>GEIRPTIGQQMETGDQRFGDLVFRQLAPNVWQHTSYLDMPGFGAVASNGLIVRDGGRVLVVDTAWTDDQTAQILNWIKQEINLPVALAVVTHAHQDKMGGMDALHAAGIATYANALSNQLAPQEGMVAAQHSLTFAANGWVEPATAPNFGPLKVFYPGPGHTSDNITVGIDGTDIAFGGCLIKDSKAKSLGNLGDADTEHYAASARAFGAAFPKASMIVMSHSAPDSRAAITHTARMADKLR[2x]

NDM-1 belongs to the B1 subclass of MBLs that requires a dinuclear metal center for full catalytic activity. Zn1 is ligated to three histidine residues, H120, H122, and H189, while Zn2 is coordinated with D124, C208, and H250. To address whether carbapenems undergo pyrroline tautomerization during hydrolysis and whether diverse protonation mechanisms exist for different β-lactams, we conduct a combined investigation on NDM-1-catalyzed hydrolysis of imipenem and meropenem using X-ray crystallography and NMR spectrometry. Our data presented here revealed informative details of the reaction including (i) double-bond tautomerization in the pyrroline ring following the cleavage of the lactam amide bond; (ii) three derivatives presumably representing EI1, EI2, and EP; (iii) absence of the bridging water molecule attributed to steric hindrance from the newly formed carboxylate that is forced to take a distinctive orientation resulting from the trans configuration of the β-lactam ring in carbapenems; and (iv) exclusive stereoselective protonation of the carbanionic intermediates.

Although both tautomers showed convergent conformations, our structures revealed two divergent modes of imipenem-zinc binding. In four imipenem- and all five meropenem-bound structures determined in this study, the carbapenem intermediates present in either Δ2 (EI1) or Δ1 (EI2) bind the dinuclear metal center in a consensus manner with hydrolyzed penicillins or cephalosporins revealed in NDM-1 strucutures. However, in the remaining two structures containing Δ1 imipenem, one oxygen atom of the C6-carboxylate (C7O) intercalates between the two Zn(II) ions, giving rise to hexahedral coordination of Zn2 with a significantly decreased C7O–Zn2 distance, from 3.2 to 2.5 Å (averaged for all imipenem copies). The imipenem molecules in these two structures show an evident shift forward to Zn2 by ~0.5 Å with respect to their counterparts in EI2, albeit remaining an almost identical overall conformation. As a result of this translational shift, the C3-carboxylate moves farther away from Zn2, markedly increasing the C3O–Zn2 distance to 3.3 Å, essentially beyond a canonical ligand-metal interacting range. Although N4 still maintains tight contact with Zn2 in this binding mode, the enzyme-intermediate interaction must be weakened due to the detachment of the C3-carboxylate from Zn2. In comparison with other imipenem-bound structures, the antibiotic molecules modeled in these two structures have significantly lower overall occupancy than the imipenem counterparts in other structures (0.74 vs. 0.89) and display higher flexibility in the R2 side chain. Considering the weakened imipenem–metal interaction and lower refined occupancy, we suppose that the species revealed in these two structures more likely represent an EP derivative in which a protonated product has been generated and is ready to be released from the active site.>[6x]MEDSNTGGTTPRNIAVLNFGTNDKKNCVTILETALYLTEKYLGKIINSSYIYETVPEYIVLDEENKIGEVTEGEPPRDISWIGDLIPTVENSRYEESEDLIYECKELEVFLKNEKINESIIREVSVEDYENEARRIIKRNDEIMKKNLEQSKDKYYTSYFFNLTVVVRTFVEDPLAMLVILKYIEQIMKRRESKKGQGEIFQNRMIDIDILFFNNYTIFEKSISLKGEDIYKIITKYIHINHTSDQNRLDIIQNLGDKIEFLCIPHVYTKYRYSILLCLNDIIPEYKHSTFEEAIRSTYNSYVESFEEKYHINIRKNNKRLYVLKDKVSYLKERTHIVGILNVNYDSFSDGGLFVDPVKAVERMFEMASDGASVIDIGGESSAPYVVPNPSVTERDLVMPVLKLFKEEWHKLECEVGGGAVCCAAASDARKNAQSSLQGKL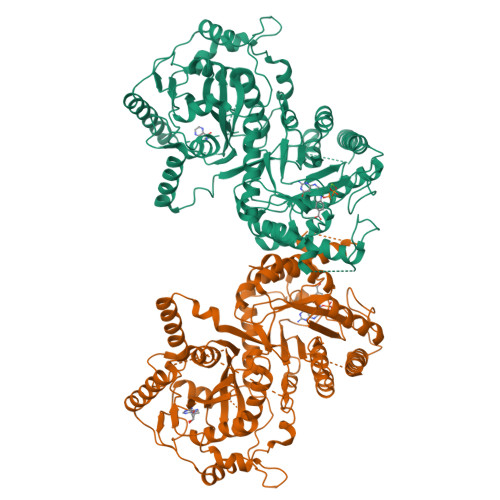QKVRDAKPIISIDTVNYDLFKECVEGELVDILNDISACTHNPEIIKLLRRKNKFYSVVLMHKRGNPHTMDKLTNYDDLISDIKRYLEDRLHFLVLNGVPRYRVLFDVGLGFAKKHDQSIKLLQHIHVYDEYPLFLGYSRKRFIVHCMGKGGAAIGECRLMSGEAKLTNGEGKLTNGEAKLTNGEGKLTNGDAKLTNGDSKLTNGEAKLTNGDPSQLWRFKMSHMRQDKDQLLYQKNICGGLAIASYSFYKKVDLIRVHDVLETKAVLDVLTRIHQP>MLDTNMKTQLRAYLEKLTKPVELIATLDDSAKSAEIKELLAEIAELSDKVTFKEDNTLPVRKPSFLITNPGSQQGPRFAGSPLGHEFTSLVLALLWTGGHPSKEAQSLLEQIRDIDGDFE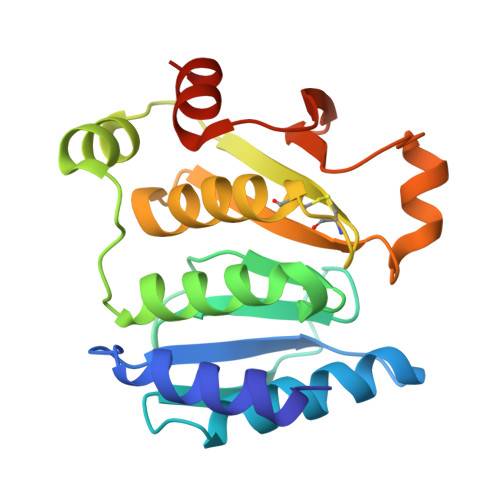FETYYSLSCHNCPDVVQALNLMAVLNPRIKHTAIDGGTFQNEITERNVMGVPAVFVNGKEFGQGRMTLTEIVAKVDTGAEKR[2x]> MWKAVMNAWNGTESQSKNVSNIQSYSFEDMKRIVGKHDPNVVLVDVR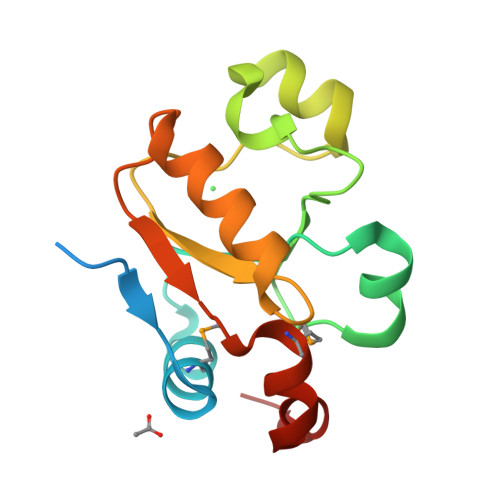EPSEYSIVHIPASINVPYRSHPDAFALDPLEFEKQIGIPKPDSAKELIFYCASGKRGGEAQKVASSHGYSNTSLYPGSMNDWVSHGGDKLDL> MTKKALSAVILAAGKGTRMYSDLPKVLHTIAGKPMVKHVIDTAHQLGSENIHLIYGHGGDLMRTHLANEQVNWVLQTEQLGTAHAVQQAAPFFKDNENIVVLYGDAPLITKETLEKLIEAKPENGIALLTVNLDNPTGYGRIIRENGNVVAIVEQKDANAEQLNIKEVNTGVMVSDGASFKKWLARVGNNNAQGEYYLTDLIALANQDNCQVVAVQATDVMEVEGANNRLQLAALERYFQNKQASKLLLEGVMIYDPARFDLRGTLEHGKDVEIDVNVIIEGNVKLGDRVKIGTGCVLKNVVIGNDVEIKPYSVLED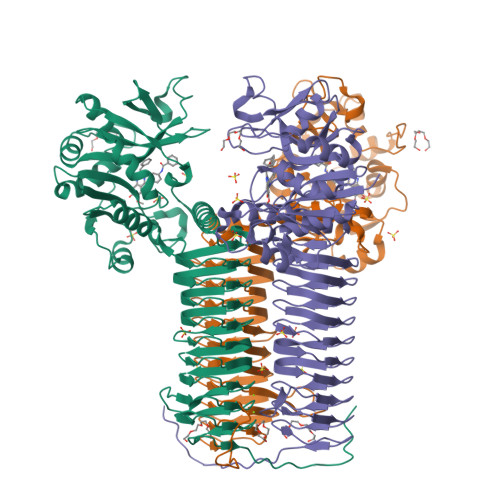SIVGEKAAIGPFSRLRPGAELAAETHVGNFVEIKKSTVGKGSKVNHLTYVGDSEIGSNCNIGAGVITCNYDGANKFKTIIGDDVFVGSDTQLVAPVKVANGATIGAGTTITRDVGENELVITRVAQRHIQGWQRPIKKK>[2x]GPHMKRYNVITIFPEMINEIFKYGVLSKGIDIGLFRVNPINLRDYTEDKHKTVDDYQYGGGHGLVMKPEPIYKAIADLKSKKDTHVVFLDPRGEQFTQKTAERLYNYDDITFVCGRYEGIDDRVRELMADEMISIGDFVITGGELAAVTIIDAVARLIPGVLGDENSPNEESFTTGLLEYPHFTRPAEFMGKKVPEVLISGNHEEIRRWRLTESIKTTLQNRPDMILRKSLSREE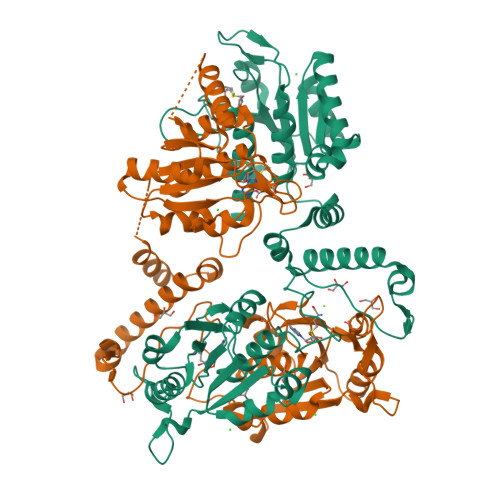EQILWSLTRGVQRKYNIYVALMHYPMRDKEGKVVTTSITNMDLHDISRSCRTFGVKNYFVVNPMPAQREIASRVVRHWIKGYGATYNENRKEAFEYTIITDSLASVIKSIEEKESGSPIIIATTARYQQKAISIEKLKEIADRPILLLFGTGWGFVDDILEFADYVLKPIHGVGDFNHLSVRSAVAIYLDRINRSFQEDIL> KHYNDGERAVLQFGKNRSEP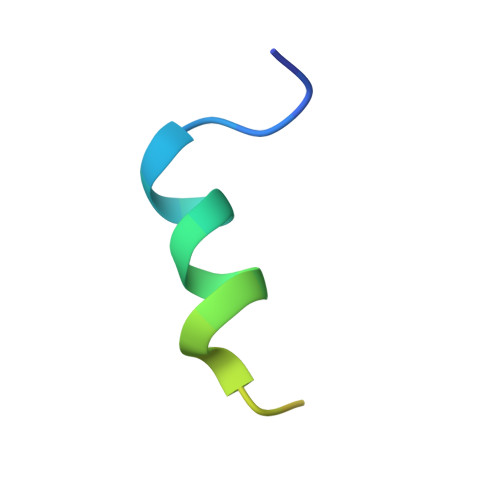IILSYKD> MEVKEVELELSSEATFLSKTSIGEITAGEKGLNPMELLLVSIGSCSGVDVYHILKKKRQEVKDIKIFLKGKRREKHPKIYEEIEIKYVAVGKVEEKALEQAVKL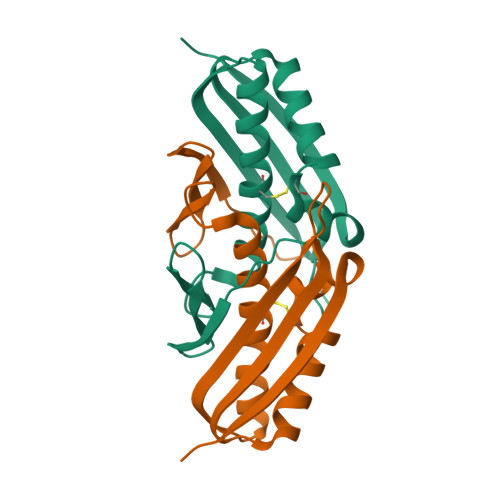STEKYCSVLAMVKPSTNLKISWEVKWEE>[12x]MFEIKKICCIGAGYVGGPTCSVIAHMCPEIRVTVVDVNESRINAWNSPTLPIYEPGLKEVVESCRGKNLFFSTNIDDAIKEADLVFISVNTPTKTYGMGKGRAADLKYIEACARRIVQNSNGYKIVTEKSTVPVRAAESIRRIFDANTKPNLNLQVLSNP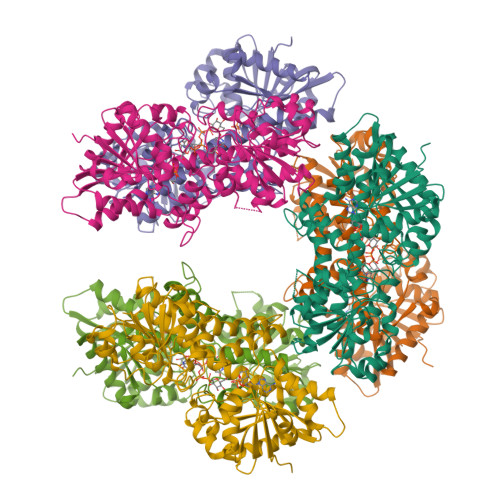EFLAEGTAIKDLKNPDRVLIGGDETPEGQRAVQALCAVYEHWVPREKILTTNTWSSELSKLAANAFLAQRISSINSISALCEATGADVEEVATAIGMDQRIGNKFLKASVGFGGSCFQKDVLNLVYLCEALNLPEVARYWQQVIDMNDYQRRRFASRIIDSLFNTVTDKKIAILGFAFKKDTGDTRESSSIYISKYLMDEGAHLHIYDPKVPREQIVVDLSHPGVSEDDQVSRLVTISKDPYEACDGAHAVVICTEWDMFKELDYERIHKKMLKPAFIFDGRRVLDGLHNELQTIGFQIETIGKKVSSKRIPYAPSGEIPKFSLQDP> MGHHHHHHHHHSSGHIDDDDKHMELFN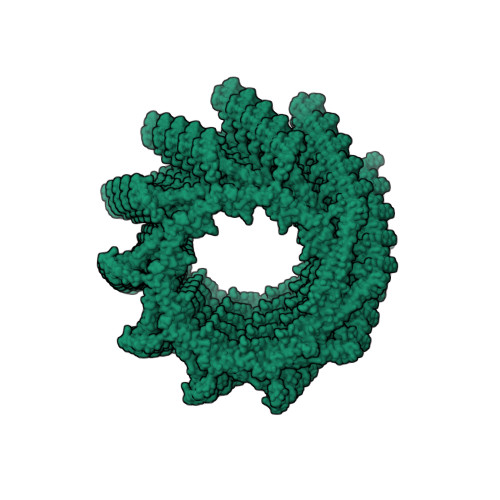RVGRVLKSQLTHWQQQQEAPEDLLERLLGEMELELIELRRALAQTIATFKSTERQRDAQQLIAQRWYEKAQAALDRGNEQLAREALGQRQSYQSHTEALGKSLGEQRALVEQVRGQLQKLERKYLELKSQKNLYLARLKSAIAAQKIEEIAGNLDNASASSLFERIETKILELEAERELLNPPPSPLDKKFEQWEEQQAVEATLAAMKARRSLPPPSS>[2x]MHHHHHHSSGRENLYFQGPGMFVQHSTAIFSDRYKGQRVLGKGSFGEVILCKDKITGQECAVKVISKRQVKQKTDKESLLREVQLLKQLDHPNIMKLYEFFEDKGYFYLVGEVYTGGELFDEIISRKRFSEVDAARIIRQVLSGITYMHKNKIVHRDLKPENLLLESKSKDANIRIIDFGLSTHFEASKKMKDKIGTAYYIAPEVLHGTYD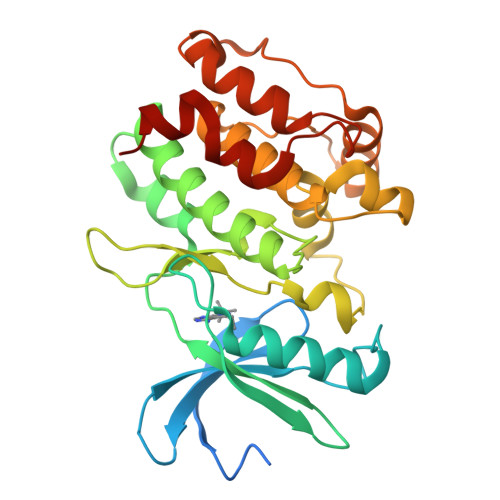EKCDVWSTGVILYILLSGCPPFNGANEYDILKKVEKGKYTFELPQWKKVSESAKDLIRKMLTYVPSMRISARDALDHEWIQTYTKEQ>[6x]SNAQTTTIHISAAASLKDSIDDVK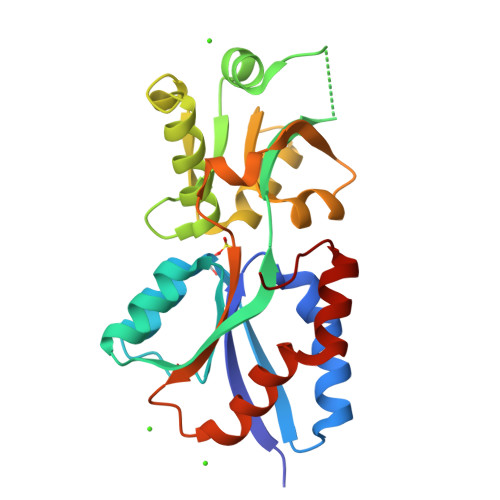PLFEKANPTIKLSFDFGGSGQIRERVESGAPIDGVLLASKKDADTLIKQNLAEKTKEFAGNELVLIEPKNVDQKTEANLEQLLNDASKIAIGDPESVPAGAYAKQTLENLNLYNAEKAKLVLATDVRQVLSYVEAGNADAGFVYQTDALLSKKVQVKAKIDEKLHDPIAYYSAQVSDSDKKEETATFLDFMNKSEAQKILEKYGFKAAN1,6-di-O-phosphono-beta-D-fructofuranose 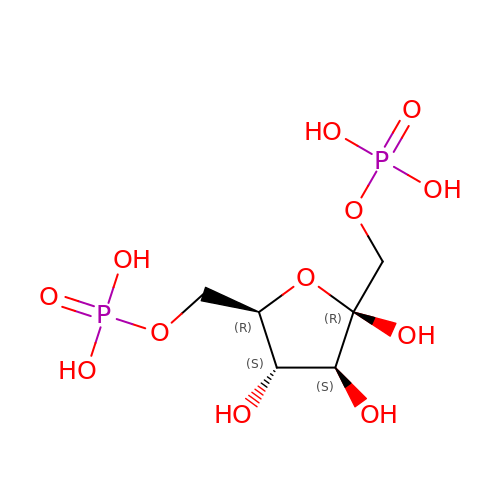| C6 H14 O12 P2 | RNBGYGVWRKECFJ-ARQDHWQXSA-N> XMDDL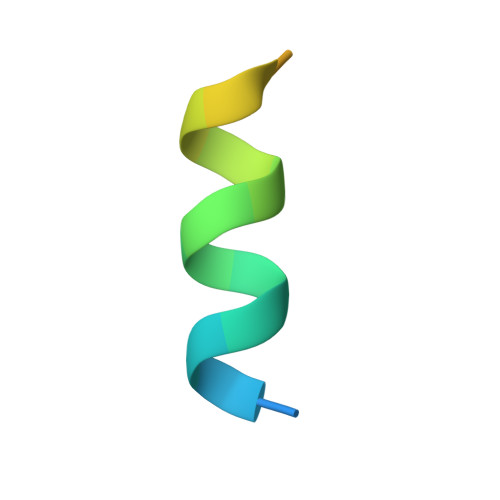DALLADLESTTSHISKX(3R,4R,5S)-4-(acetylamino)-5-amino-3-(pentan-3-yloxy)cyclohex-1-ene-1-carboxylic 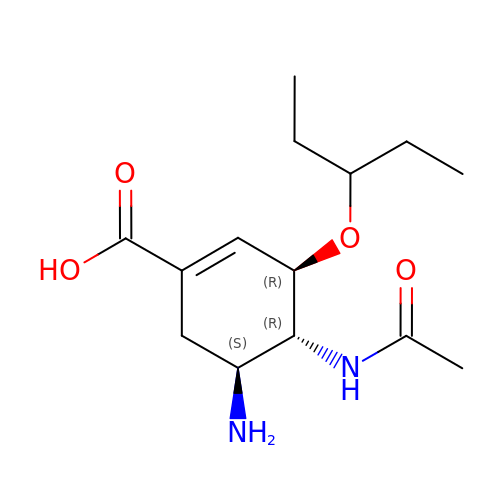acid | C14 H24 N2 O4 | NENPYTRHICXVCS-YNEHKIRRSA-N> SVAVQLQYDPVYDNADQSFGTVACSDGPNGMLTKGYSTFGSVPSYVGAVDTIT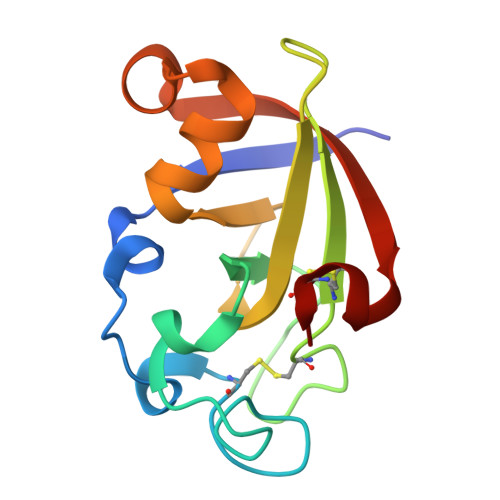GWNSESCGTCYQITWSGTGKTIHVVGVDVAGNGFNVGQRAMDDLTNGQAVALGNIDVTATLVDKSACRL> MAPTSSIEIVLDKTTASVGEI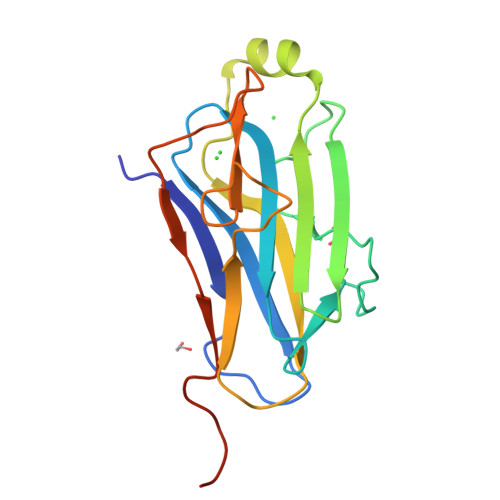VTASINIKNITNFSGCQLNMKYDPAVLQPVTSSGVAYTKSTMPGAGTILNSDFNLRQVADNDLEKGILNFSKAYVSLDDYRTAAAPEQTGTVAVVKFKVLKEETSSISFEDTTSVPNAIDGTVLFDWNGDRIQSGYSVIQPAVINLDMIKASLEHHHHHH> SSQIRQNYSTEVEAAVNRLVNLYLRASYTYLSLGFYFDRDDVALEGVCHFFRELAEEKREGAERLLKMQNQRGGRALFQDLQKPSQDEWGTTPDAMKAAIVLEKSLNQALLDLAALGSAQADPHLCDFLESHFLDEEVKLIKKMGDHLTNIQR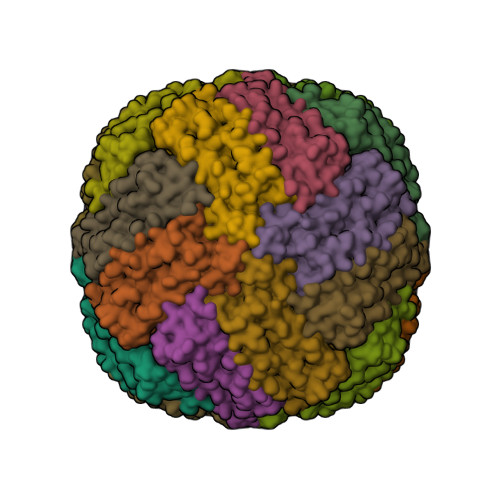LVGSQAGLGEYLFERLTLKHD> SSHHHHHHMSGENLYFQGASAAIVTDTGGVDDKSFNQSAWEGLQAW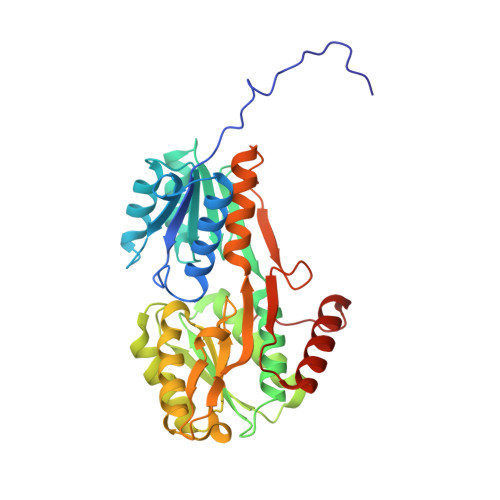GKEHNLSKDNGFTYFQSTSEADYANNLQQAAGSYNLIFGVGFALNNAVKDAAKEHTDLNYVLIDDVIKDQKNVASVTFADNESGYLAGVAAAKTTKTKQVGFVGGIESEVISRFEAGFKAGVASVDPSIKVQVDYAGSFGDAAKGKTIAAAQYAAGADIVYQVAGGTGAGVFAEAKSLNESRPENEKVWVIGVDRDQEAEGKYTSKDGKESNFVLVSTLKQVGTTVKDISNKAERGEFPGGQVIVYSLKDKGVDLAVTNLSEEGKKAVEDAKAKILDGSVKVPEK> GAMETRLNVVLRGIAFGARPGAVIEEGGKQ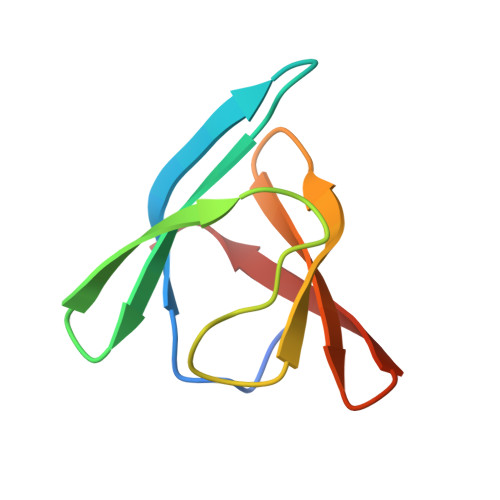QVYLQGERLDSHNAVIEEINRDHVMLRYQGKIERLSLA>[3x]TEGSSKPRVAVTTSFLNDMVYQLAGDEVERDLLIPAGEDPHLYVAKSSDLSKLQKADLVLYHGLHFEGKMVEALEKTGVAVSKNFNAKDLNTMDEDGEEIVDPHFWFSIPLYKSAVAVASEELQKLLPAKAEMIQKNTEKYQAQLDDLHAWVEKELSVIPKESRYLVTPHDAFNYFAASYDFTLYAPQGVSTDSEVANSDMIETVNLIID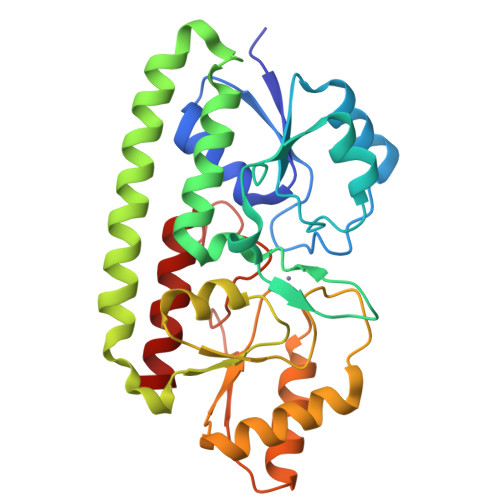HNIKAIFTESTTNPERMKKLQEAVKAKGGQVEVVTGEGKELFSDSLAPEGEEGDTFIDMYKHNVKLMVKYLK>[60x]MKAFEFLYEDFQRGLTVVLDKGLPPKFVEDYLKVCGDYIDFVKFGWGTSAVIDRDVVKEKINYYKDWGIKVYPGGTLFEYAYSKGEAAEFIAECKKLGFEAVEISDGSSDISLDDRKAAIWGAKWAGFMVLTEVGKKMPDKDKQLTIDDRIKLINFDLDAGADYVIIEGRESGKGIGLFDKEGKVKENELDVLAKNVDINKVIFEAPQKSQQVAFILKFGSSVNLANIAFDEVISLETLRRGLRGDT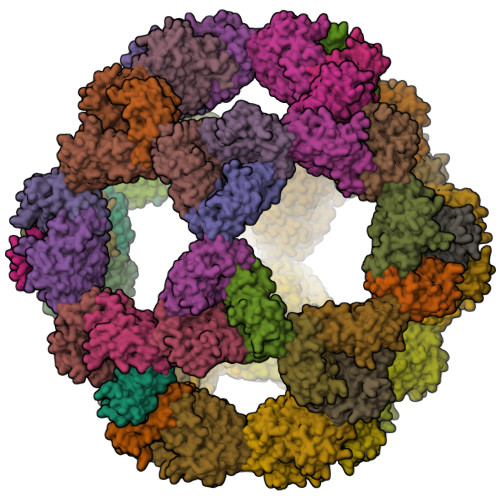FGKVLEHHHHHH>NYEKLKNRLVQNARVAARQKEYTEIPDIFLCPISKTLIKTPVITAQGKVYDQEALSNFLIATGNKDETGKKLSIDDVVVFDELYQQIKVYNF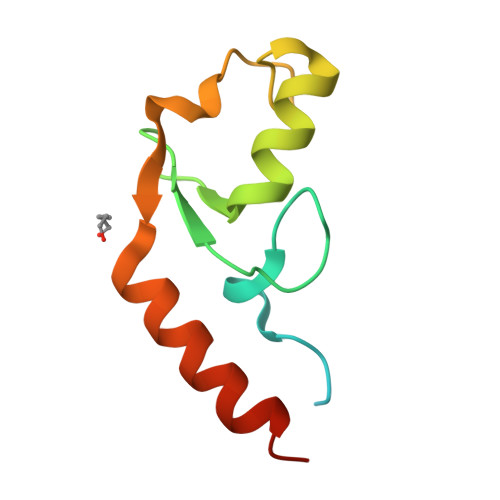YRKREVQKN[3x]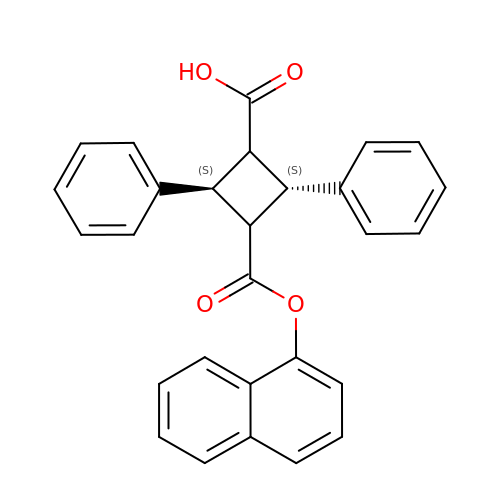(1S,2S,3S,4S)-3-{[(naphthalen-1-yl)oxy]carbonyl}-2,4-diphenylcyclobutane-1-carboxylic acid | C28 H22 O4 | NVOKBONTLOAJKA-CQJMVLFOSA-N> LVHVASVEKGRSYEDFQKVYNAIALKLREDDEYDNYIGYGPVLVRLAWHISGTWDKHDNTGGSYGGTYRFKKEFNDPSNAGLQNGFKFLEPIHKEFPWISSGDLFSLGGVTAVQEMQGPK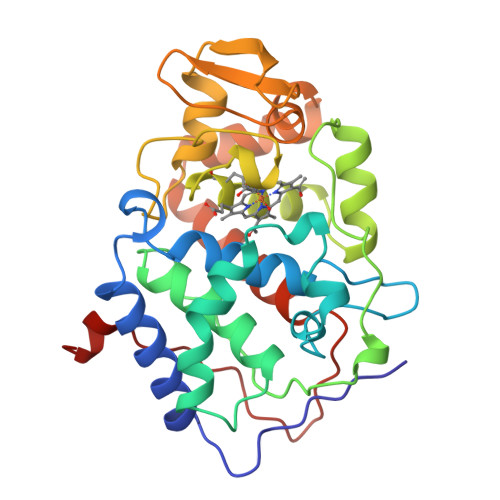IPWRCGRVDTPEDTTPDNGRLPDADKDAGYVRTFFQRLNMNDREVVALMGAHALGKTHLKNSGYEGPWGAANNVFTNEFYLNLLNEDWKLEKNDANNEQWDSKSGYMMLPTDYSLIQDPKYLSIVKEYANDQDKFFKDFSKAFEKLLEDGITFPKDAPSPFIFKTLEEQGL>TRDQNGTWEMESNENFEGYMKALDIDFATRKIAVRLTQTLVIDQDGDNFKTKATSTFFNYDVDFTVGVEFDEYTKSLDNRHVKALVTWEGDVLVCVQKGEKENRGWKKWIEGDKLYLELTCGDQVCRQVFKKK[4x]

Human cellular retinol binding protein II (hCRBPII) was used as a protein engineering platform to rationally regulate absorptive and emissive properties of a covalently bound fluorogenic dye. We demonstrate the binding of a thio-dapoxyl analog via formation of a protonated imine between an active site lysine residue and the chromophore’s aldehyde. Previously, we showed the utility of human cellular retinol-binding protein II (hCRBPII) mutants as a fluorophoric tag, wherein an active site lysine residue (Q108K) reacts with synthetic aldehydic chromophores, giving rise to the formation of either an imine (Schiff base, SB) or an iminium (protonated SB, PSB). Q108K functions as the active-site lysine and forms a Schiff base with the aldehyde, whereas the K40L mutation is assumed to eliminate interactions between Q108K and Lys40, an interaction that could otherwise impede imine formation, and is also required to promote Schiff base protonation.

Subsequently, our investigation aimed to alter the polarity of the Thr53 position, which makes a water mediated hydrogen bond with Thr51 in crystal structures where both residues are maintained. The T53A mutation also red-shifted absorption and emission, but far more modestly (5 and 3 nm respectively, compare M4 to M1). We next turned our attention to the entrance to the binding pocket because our previous studies with retinal showed that introduction of aromatic residues in this region leads to the closure of the binding pocket and results in substantial bathochromic shifts.>[4x]XNRVFAEYPDHIQD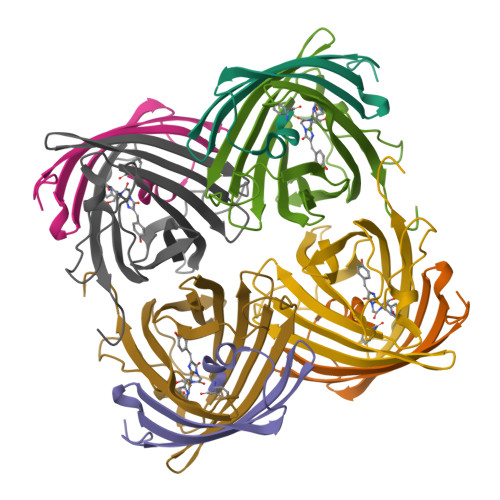YFKQSFPKGYSWERSLTFEDGGICIARNDITMEGDTFYNKVRFHGVNFPANGPVMQKKTLKWEPSTEKMYVRDGVLTGDITMALLLEGNAHYRCDFRTTYKAKEKGVKLPGYHFVDHCIEILSHDKDYNKVKLYEHAVAHSGLPD;>GGAIKPDMKINLRMEGNVNGHHFVIDGDGTGKPFEGKQSMDLEVKEGGPLPFAFDILTTAF[4x]>[4x]MNPNQKIITIGSVSLTIATVCFLMQIAILATTVTLHFKQHECDSPASNQVMPCEPIIIERNITEIVYLNNTTIEKEICPKVVEYRNWSKPQCQITGFAPFSKDNSIRLSAGGDIWVTREPYVSCDPGKCYQFALGQGTTLDNKHSNDTVHDRIPHRTLLMNELGVPFHLGTRQVCIAWSSSSCHDGKAWL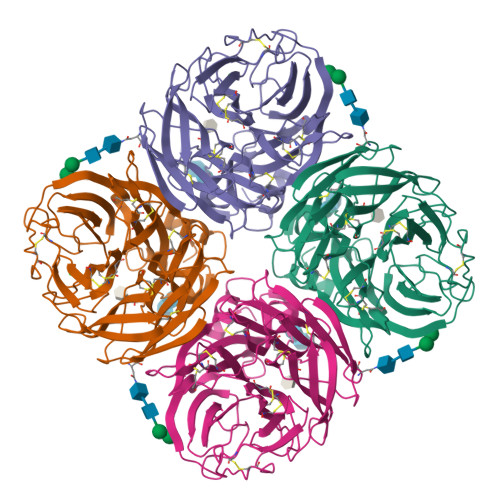HVCITGDDKNATASFIYDGRLVDSIGSWSQNILRTQESECVCINGTCTVVMTDGSASGRADTRILFIEEGKIVHISPLSGSAQHIEECSCYPRYPGVRCICRDNWKGSNRPVVDINMEDYSIDSSYVCSGLVGDTPRNDDSSSNSNCRNPNNERGTQGVKGWAFDNGNDLWMGRTISKESRSGYETFKVIGGWSTPNSKSQVNRQVIVDNNNWSGYSGIFSVEGKSCINRCFYVELIRGRPQETRVWWTSNSIVVFCGTSGTYGTGSWPDGANINFMPI> SMEVFQNHFEPGVY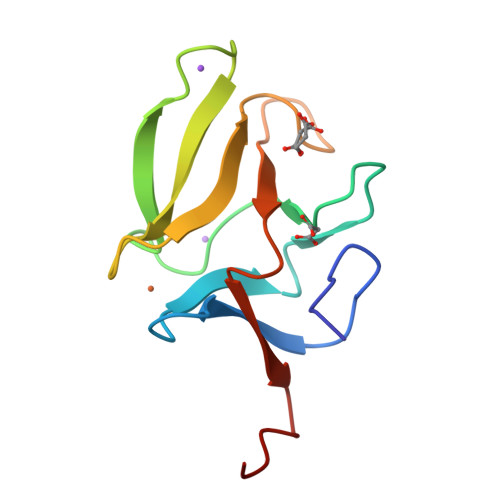VCAKCGYELFSSRSKYAHSSPWPAFTETIHADSVAKRPEHNRSEALKVSCGKCGNGLGHEFLNDGPKPGQSRFSIFSSSLKFVPKGKETSA> XGGKWSKSSVIGWPAVRERMRRAEPAADGVGAASRDLEKHGAITSSNTAANNAACAWLEAQEEEKVGFPVTPQVPLRPMTYKAAVDLSHFLKEKGGLEGLIHSQRRQDILDL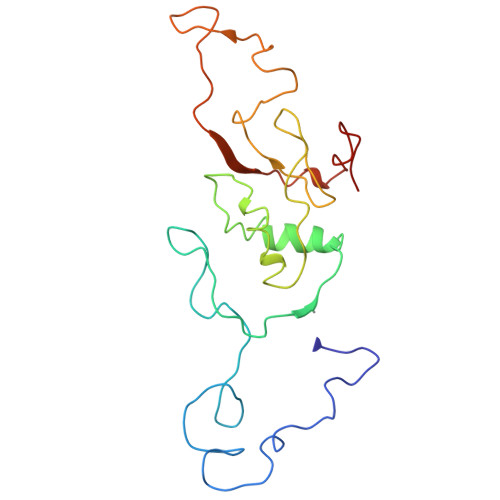WIYHTQGYFPDWQNYTPGPGIRYPLTFGWCYKLVPVEPDKVEEANKGENTSLLHPVSLHGMDDPEREVLEWRFDSRLAFHHVARELHPEYFKNC>GSHMKVMFIPSRAVPFNPDRVQGGLEAVHLNVLKYLVSIGADIDYIGFDNDTFGDWKVTHHPVGHLTKFSLGMSYTMARKIVELAGIHEYDFVVTMEPTKLTVQAIKDAGLSKVHKNFMATPFEPVSRGIVQIWDQTIQIHKNGGKSYAPTKAFREFERKYCHMTSALTDKIDYDYWRANPLFEAEDYPVICLNEKPEVLPATDLIISAQRYDTKMRRTDVALEAIKALGENGVGYCPSKWAPPAKYPVIIDAPHSEIMERLKTAKALINTCPDTGTVENSSIEAISKGVPVIQLVFKDYPHATFEYDPDTVRVEIDFSTPKK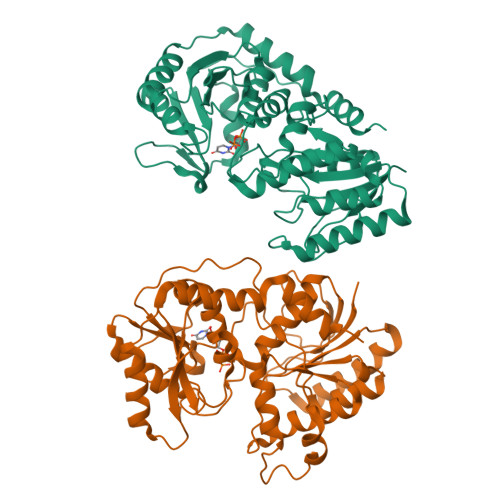EVVALYTKAVLEFTDTYEARVKRAEAVWKKYNRDAVVAMWDKIFTA[2x]>MKLNIRAQTAQNQHNNSPIVLVHGLFGSLDNLGVLARDLVNDHNIIQVDVRNHGLSPREPVMNYPAMAQDLVDTLDAQQIDKATFIGHS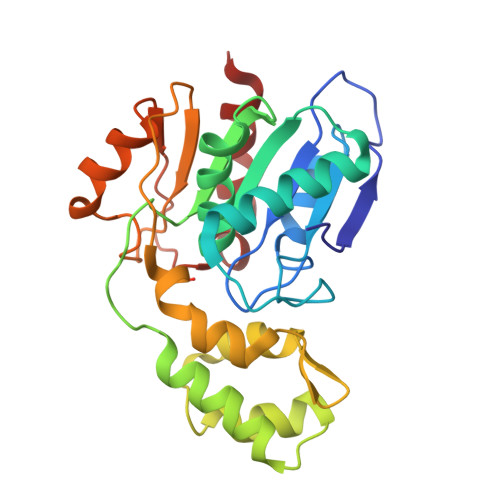MGGKAVMALTALAPDRIDKLVAIDIAPVDYHVRRHDEIFAAINAVSESDAQTRQQAAAIMRQHLNEEGVIQFLLKSFVDGEWRFNVPVLWDQYPHIVGWEKIPAWDHPALFIPGGNSPYVSEQYRDDLLAQFPQARAHVIAGAGHWVHAEKPDAVLRAIRRYLNDH[2x]> MASWSHAPKFEKGASLDSPTFGCTDSPVRRERGQKAVFCGLTSIVWLHRKMQDAFFLVVGSRTCAHLLQAAAGVMIFAEPRFGTAVLEEQDLAGLADAHKELDREVAKLLERRPDIRQLFLVGSCPSEVLKLDLDRAAERLSGLHAPHVRVYSYTGSGLDTTFTQGEDTCLAAMVPTLDTTEAAELIVVGALPDVVEDQCLSLLTQLGVGPVRMLPARRSDIEPAVGPNTRFILAQPFLGETTGALERRGAKRIAAPFPFGEEGTTLWLKAVADAYGVSAEKFEAVTAAPRARAKKAIAAHLETLTGKSLFMFPDSQLEIPLARFLARECGMKTTEIATPFLHKAIMAPDLALLPSNTALTEGQDLEAQLDRHEAIN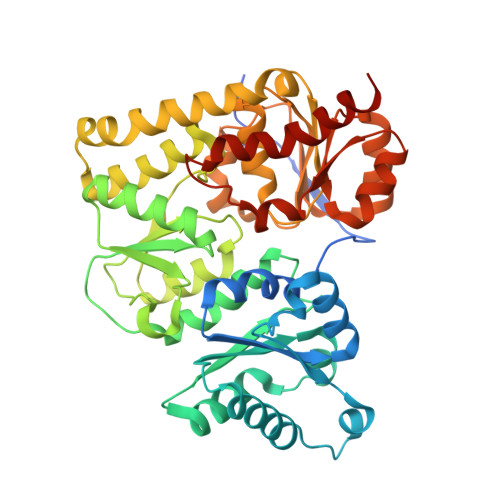PDLTVCGLGLANPLEAKGHATKWAIELVFTPVHFYEQAGDLAGLFSRPLRRRALLNGGAA> MLTSERSYLRYPKNRRWTEAGRFWAPHPENVLFIHKPTMEETRRVALGLRSQLVRNRERKTKAHLLSLELDRLVQVHDSRVRVINADIDAVKQMIGNMTWSDNIDMPQSRSHEPPLVTSPPQASHRNFTVAIVPGDPHFSVDRDLRGELMPTLYMNQNQWLPSFGPWFISLTDNAMQRRVFPKELKGTVNFQNSTSLKLISHTLTTVASTTADFFADARHLTDTQAALCLVNAYFCQKTSRQLPATPDDLLADLPQKLDLLITQLKQESGPGDFSFTYSNPQERASLAPLNKESRYPTAFFQRHKLHAMMAKAGLFPHNKGTGAPGTAPAMDLVFAITSAMFGSDIPPFSAYQWNLRAGIVALEVFILAYGLLEFGQVARGHPNRRLNLVSLLGPKFQPGALPDPNAPMLKRGQLFSFISEHYIIPTLQANPNAPVSFIFP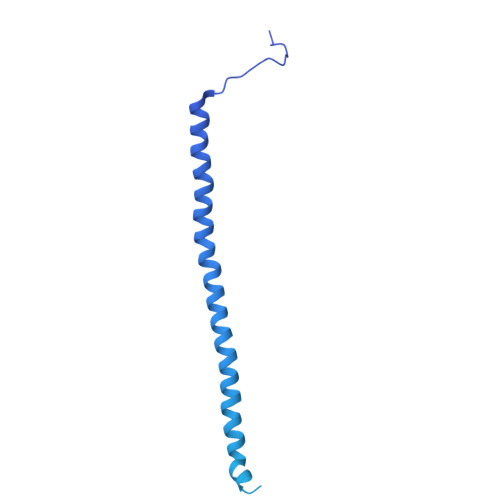GIILAALEARSTVSHKQPGPFVNLTGSRFNEIFEILNQQLTFRDPLALLQARTALRLATEEGLDVLLSHPSPPTLLQEIIKSQFGGGDDYDRAYFMVLGCLPVVLAVV>[4x]DMRPEIWIAQELRRI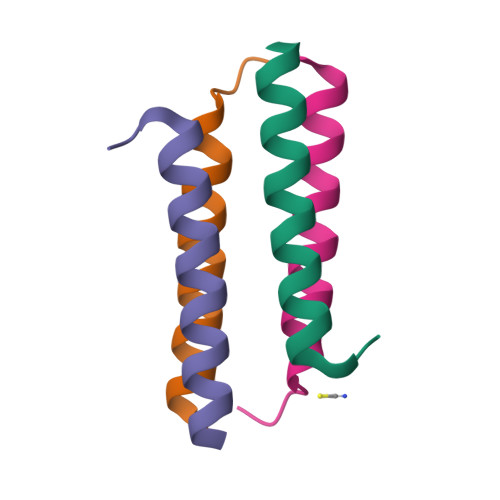GDEFNAYYARRX> AQYEDGKQYTTLEKPVAGAPQVLEFFSFFCPHAYQFEEVLHISDNVKKKLPEGVKMTKYHVNFMGGDLGKDLTQAWAVAMALGVEDKVTVPLFEGVQKTQTIRSASDIRDVFINAGIKGEEYDAAWNSFVVKSLVAQQEKAAADVQLRGVPAMFVNGKYQLNPQGMDTSNMDVFVQQYADTVKYLSEKK;> MLRFLNQASQGRGAWLLMAFTALALELTALWFQHV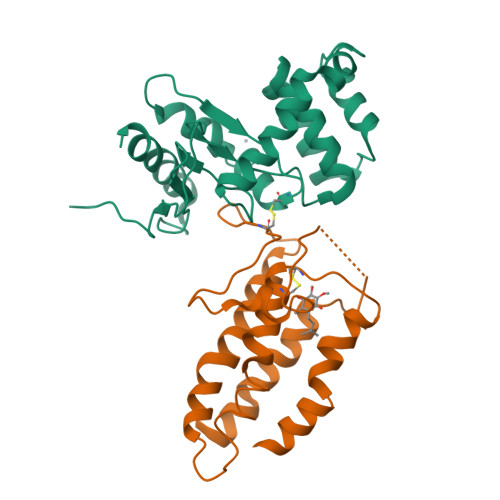MLLKPCVLCIYERVALFGVLGAALIGAIAPKTPLRYVAMVIWLYSAFRGVQLTYEHTMLQLYPSPFATCDFMVRFPEWLPLDKWVPQVFVASGDSAERQWDFLGLEMPQWLLGIFIAYLIVAVLVVISQPFKAKKRDLFGR>[2x]MMEQVCDVFDIYAICACCKVESKNEGKKNEVFNNYTFRGLGNKGVLPWKCNSLDMKYFCAVTTYVNESKYEKLKYKRCKYLNKETVDNVNDMPNSKKLQNVVVMGRTSWESIPKKFKPLSNRINVILSRTLKKEDFDEDVYII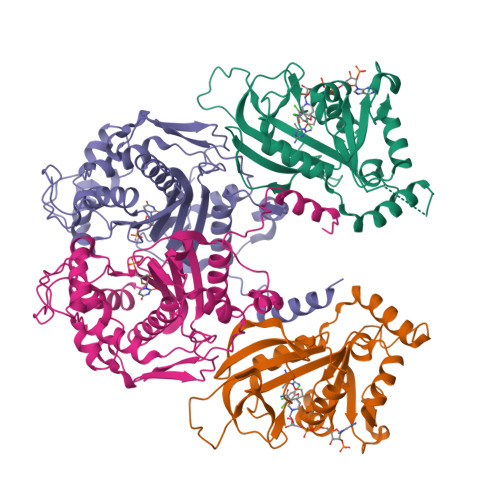NKVEDLIVLLGKLNYYKCFIIGGSVVYQEFLEKKLIKKIYFTRINSTYECDVFFPEINENEYQIISVSDVYTSNNTTLDFIIYKKTNNKMLNEQNCIKGEEKNNDMPLKNDDKDTCHMKKLTEFYKNVDKYKINYEN;>[2x]DDDDEEEDDFVYFNFNKEKEEKNKNSIHPNDFQIYNSLKYKYHPEYQYLNIIYDIMMNGNKQSDRTGVGVLSKFGYIMKFDLSQYFPLLTTKKLFLRGIIEELLWFIRGETNGNTLLNKNVRIWEANGTREFLDNRKLFHREVNDLGPIYGFQWRHFGAEYTNMYDNYENKGVDQLKNIINLIKNDPTSRRILLCAWNVKDLDQMALPPCHILCQFYVFDGKLSCIMYQRSCDLGLGVPFNIASYSIFTHMIAQVCNLQPAQFIHVLGNAHVYNNHIDSLKIQLNRIPYPFPTLKLNPDIKNIEDFTISDFTIQNYVHHEKISMDMAA>MGSSHHHHHHSSGRENLYFQGMRSTSYYPVIMTSDVAATAAFYCQHFGFRPLFEADWYVHLQSAEDPAVNLAILDGQHSTIPAAGRGQVSGLILNFEVDDPDREYARLQQAGLPILLTLRDE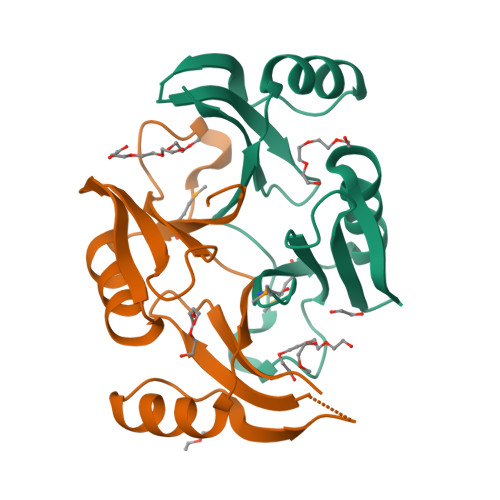DFGQRHFITADPNGVLIDIIKPIPPSANYAAQYAGGAAAAQP[2x]> MLGTGPAAATTAATTSSNVSVLQQFASGLKSRNEETRAKAAKELQHYVTMELREMSQEESTRFYDQLNHHIFELVSSSDANERKGGILAIASLIGVEGGNATRIGRFANYLRNLLPSNDPVVMEMASKAIGRLAMAGDTFTAEYVEFEVKRALEWLGADRNEGRRHAAVLVLRELAISVPTFFFQQVQPFFDNIFVAVWDPKQAIREGAVAALRACLILTTQREPKEMQKPQWYRHTFEEAEKGFDETLAKEKGMNRDDRIHGALLILNELVRISSMEGERLREEMEEITQQQLVHDKYCKDLMGFGTKPRHITPFTSFQAVQPQQSNALVGLLGYSSHQGLMGFGTSPSPAKSTLVESRCCRDLMEEKFDQVCQWVLKCRNSKNSLIQMTILNLLPRLAAFRPSAFTDTQYLQDTMNHVLSCVKKEKERTAAFQALGLLSVAVRSEFKVYLPRVLDIIRAALPPKDFAHKRQKAMQVDATVFTCISMLARAMGPGIQQDIKELLEPMLAVGLSPALTAVLYDLSRQIPQLKKDIQDGLLKMLSLVLMHKPLRHPGMPKGLAHQLASPGLTTLPEASDVGSITLALRTLGSFEFEGHSLTQFVRHCADHFLNSEHKEIRMEAARTCSRLLTPSIHLISGHAHVVSQTAVQVVADVLSKLLVVGITDPDPDIRYCVLASLDERFDAHLAQAENLQALFVALNDQVFEIRELAICTVGRLSSMNPAFVMPFLRKMLIQILTELEHSGIGRIKEQSARMLGHLVSNAPRLIRPYMEPILKALILKLKDPDPDPNPGVINNVLATIGELAQVSGLEMRKWVDELFIIIMDMLQDSSLLAKRQVALWTLGQLVASTGYVVEPYRKYPTLLEVLLNFLKTEQNQGTRREAIRVLGLLGALDPYKHKVNIGMIDQSRDASAVSLSESKSSQDSSDYSTSEMLVNMGNLPLDEFYPAVSMVALMRIFRDQSLSHHHTMVVQAITFIFKSLGLKCVQFLPQVMPTFLNVIRVCDGAIREFLFQQLGMLVSFVKSHIRPYMDEIVTLMREFWVMNTSIQSTIILLIEQIVVALGGEFKLYLPQLIPHMLRVFMHDNSPGRIVSIKLLAAIQLFGANLDDYLHLLLPPIVKLFDAPEAPLPSRKAALETVDRLTESLDFTDYASRIIHPIVRTLDQSPELRSTAMDTLSSLVFQLGKKYQIFIPMVNKVLVRHRINHQRYDVLICRIVKGYTLADEEEDPLIYQHRMLRSGQGDALASGPVETGPMKKLHVSTINLQKAWGAARRVSKDDWLEWLRRLSLELLKDSSSPSLRSCWALAQAYNPMARDL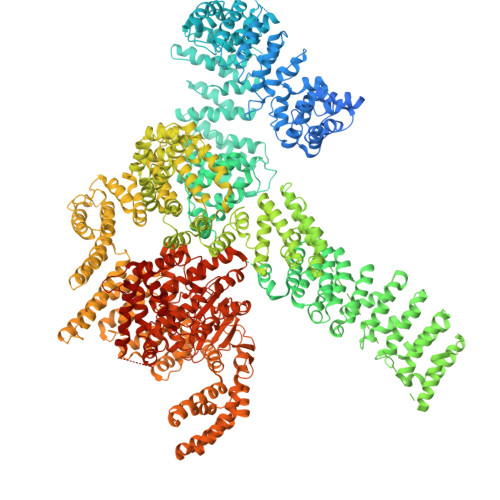FNAAFVSCWSELNEDQQDELIRSIELALTSQDIAEVTQTLLNLAEFMEHSDKGPLPLRDDNGIVLLGERAAKCRAYAKALHYKELEFQKGPTPAILESLISINNKLQQPEAAAGVLEYAMKHFGELEIQATWYEKLHEWEDALVAYDKKMDTNKDDPELMLGRMRCLEALGEWGQLHQQCCEKWTLVNDETQAKMARMAAAAAWGLGQWDSMEEYTCMIPRDTHDGAFYRAVLALHQDLFSLAQQCIDKARDLLDAELTAMAGESYSRAYGAMVSCHMLSELEEVIQYKLVPERREIIRQIWWERLQGCQRIVEDWQKILMVRSLVVSPHEDMRTWLKYASLCGKSGRLALAHKTLVLLLGVDPSRQLDHPLPTVHPQVTYAYMKNMWKSARKIDAFQHMQHFVQTMQQQAQHAIATEDQQHKQELHKLMARCFLKLGEWQLNLQGINESTIPKVLQYYSAATEHDRSWYKAWHAWAVMNFEAVLHYKHQNQARDEKKKLRHASGANITNATTAATTAATATTTASTEGSNSESEAESTENSPTPSPLQKKVTEDLSKTLLMYTVPAVQGFFRSISLSRGNNLQDTLRVLTLWFDYGHWPDVNEALVEGVKAIQIDTWLQVIPQLIARIDTPRPLVGRLIHQLLTDIGRYHPQALIYPLTVASKSTTTARHNAANKILKNMCEHSNTLVQQAMMVSEELIRVAILWHEMWHEGLEEASRLYFGERNVKGMFEVLEPLHAMMERGPQTLKETSFNQAYGRDLMEAQEWCRKYMKSGNVKDLTQAWDLYYHVFRRISKQLPQLTSLELQYVSPKLLMCRDLELAVPGTYDPNQPIIRIQSIAPSLQVITSKQRPRKLTLMGSNGHEFVFLLKGHEDLRQDERVMQLFGLVNTLLANDPTSLRKNLSIQRYAVIPLSTNSGLIGWVPHCDTLHALIRDYREKKKILLNIEHRIMLRMAPDYDHLTLMQKVEVFEHAVNNTAGDDLAKLLWLKSPSSEVWFDRRTNYTRSLAVMSMVGYILGLGDRHPSNLMLDRLSGKILHIDFGDCFEVAMTREKFPEKIPFRLTRMLTNAMEVTGLDGNYRITCHTVMEVLREHKDSVMAVLEAFVYDPLLNWRLMDTNTKGNKRSRTRTDSYSAGQSVEILDGVELGEPAHKKTGTTVPESIHSFIGDGLVKPEALNKKAIQIINRVRDKLTGRDFSHDDTLDVPTQVELLIKQATSHENLCQCYIGWCPFW>[6x]MVKLENSRKPEKISNKNIPMSDFVVNLDHGDPTAYEEYWR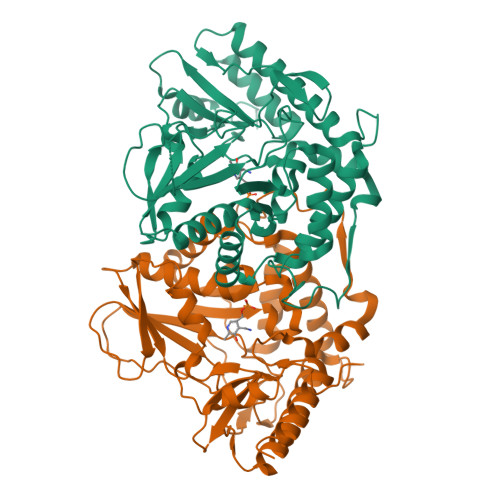KMGDRCTVTIRGCDLMSYFSDMTNLCWFLEPELEDAIKDLHGVVGNAATEDRYIVVGTGSTQLCQAAVHALSSLARSQPVSVVAAAPFYSTYVEETTYVRSGMYKWEGDAWGFDKKGPYIELVTSPNNPDGTIRETVVNRPDDDEAKVIHDFAYYWPHYTPITRRQDHDIMLFTFSKITGHAGSRIGWALVKDKEVAKKMVEYIIVNSIGVSKESQVRTAKILNVLKETCKSESESENFFKYGREMMKNRWEKLREVVKESDAFTLPKYPEAFCNYFGKSLESYPAFAWLGTKEETDLVSELRRHKVMSRAGERCGSDKKHVRVSMLSREDVFNVFLERLANMKLIKSIDL> GPTPASYNLAVRRAAPAVVNVYNRGLNTNSHNQLEIRTLGSGV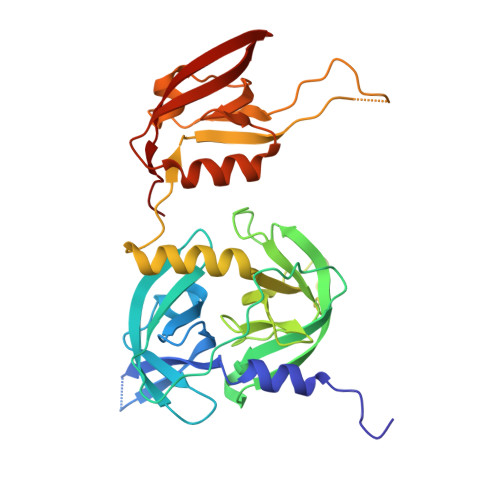IMDQRGYIITNKHVINDADQIIVALQDGRVFEALLVGSDSLTDLAVLKINATGGLPTIPINARRVPHIGDVVLAIGNPYNLGQTITQGIISATGRIGLNPTGRQNFLQTDASINHGNSGGALVNSLGELMGINTLSFDKSNDGETPEGIGFAIPFQLATKIMDKLIRDGRVIRGYIGIGGREIAPLHAQGGGIDQLQGIVVNEVSPDGPAANAGIQVNDLIISVDNKPAISALETMDQVAEIRPGSVIPVVVMRDDKQLTLQVTIQEYPATN>MAHHHHHHHRSEQIAAVRRMVEAYNTGKTDDVADYIHPEYMNPGTLEFTSLRGPELFAINVAWVKKTFSEEARLEEVGIEERADWVRARLVLYGRHVGEMV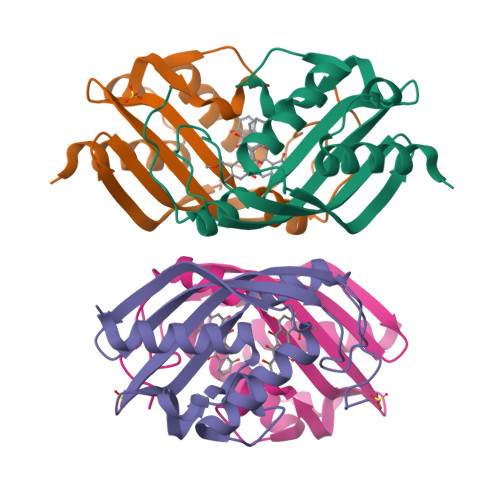GMAPTGRLFSGEQIHLLHFVDGKIHHHRDWPDYQGTYRQLGEPWPETEHRRP[4x]> SELQTEGRTRYHGRNVCSTWGNFHYKTFDGDVFRFPGLCDYNFASDCRGSYKEFAVHLKRGPGQAEAPAGVESILLTIKDDTIYLTRHLAVLNGAVVSTPHYSPGLLIEKSDAYTKVYSRAGLTLMWNREDALMLELDTKFRNHTCGLCGDYNGLQSYSEFLSDGVLFSPLEFGNMQKINQPDVVCEDPEEEVAPASCSEHRAECERLLTAEAFADCQDLVPLEPYLRACQQDRCRCPGGDTCVCSTVAEFSRQCSHAGGRPGNWRTATLCPKTCPGNLVYLESGSPCMDTCSHLEVSSLCEEHRMDGCFCPEGTVYDDIGDSGCVPVSQCHCRLHGHLYTPGQEITNDCEQCVCNAGRWVCKDLPCPGTCALEGGSHITTFDGKTYTFHGDCYYVLAKGDHNDSYALLGELAPCGSTDKQTCLKTVVLLADKKKNAVVFKSDGSVLLNQLQVNLPHVTASFSVFRPSSYHIMVSMAIGVRLQVQLAPVMQLFVTLDQASQGQVQGLCGNFNGLEGDDFKTASGLVEATGAGFANTWKAQSTCHDKLDWLDDPCSLNIESANYAEHWCSLLKKTETPFGRCHSAVDPAEYYKRCKYDTCNCQNNEDCLCAALSSYARACTAKGVMLWGWREHVCNKDVGSCPNSQVFLYNLTTCQQTCRSLS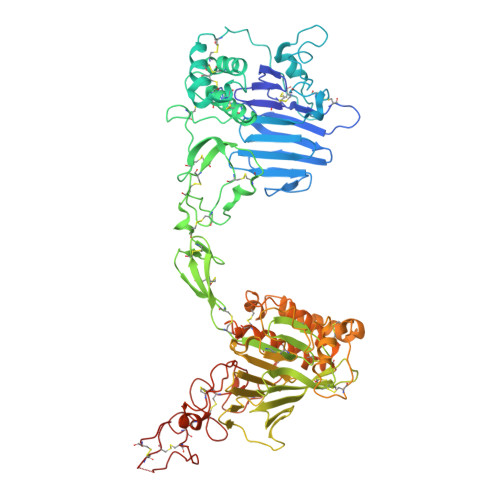EADSHCLEGFAPVDGCGCPDHTFLDEKGRCVPLAKCSCYHRGLYLEAGDVVVRQEERCVCRDGRLHC> VEMVDNLRGKSGQGYYVEMTVGSPPQTLNILVDTGSSNFAVGAAPHPFLHRYYQRQLSSTYRDLRKGVYVPYTQGKWEGELGTDLVSIPHGPNVTVRANIAAITESDKFFINGSNWEGILGLAYAEIARPDDSLEPFFDSLVKQTHVPNLFSLQLCGAGFPLNQSEVLASVGGSMIIGGIDHSLYTGSLWYTPIRREWYYEVIIVR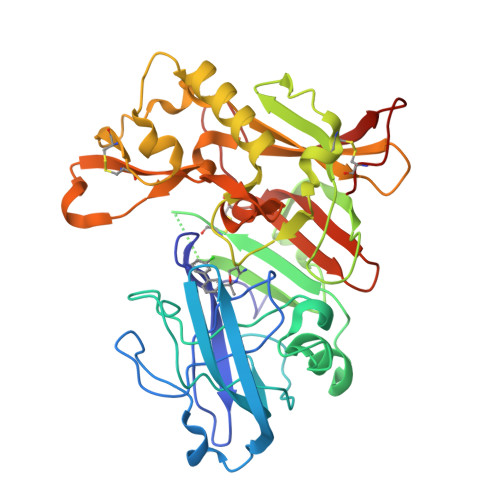VEINGQDLKMDCKEYNYDKSIVDSGTTNLRLPKKVFEAAVKSIKAASSTEKFPDGFWLGEQLVCWQAGTTPWNIFPVISLYLMGEVTNQSFRITILPQQYLRPVEDVATSQDDCYKFAISQSSTGTVMGAVIMEGFYVVFDRARKRIGFAVSACHVHDEFRTAAVEGPFVTLDMEDCGY Magnaporthe oryzae, a fungal pathogen of rice blast, is the most devastating rice pathogen and causes a destructive decrease in rice production in epidemic years. MoHrip2, a novel elicitor isolated from M. oryzae, is an exocrine protein. In our previous work, we showed that MoHrip2 causes necrotic lesions and triggers early signaling events in the tobacco leaf defense system, and we showed that MoHrip2 also enhanced resistance to M. oryzae in rice. Although, the MoHrip2 amino acid sequence showed up to 70% similarity to several specific plant fungal pathogen proteins, the specific function of both MoHrip2 and proteins with similar sequences are unknown.

In this study, we solved the crystal structure of MoHrip2 by X-ray crystallography using the single-wavelength anomalous dispersion (SAD) method. There were two identical protein molecules in an asymmetric unit, and only one monomer is shown. The overall architecture is a β-barrel consisting of 11 β-sheets and a very short α-helix. The short helix was located between the β9 and β10 sheet. MoHrip2 contains six cysteines that are involved in three intramolecular disulfide bridges, which occur between cysteines 27 and 151, 116 and 140, and 121 and 129. On the basis of the crystal structure, MoHrip2 showed a high similarity to the three-dimensional structure of a large family of proteins containing a thaumatin-like domain despite the low homology of their primary sequences. Of these proteins, we were interested in xylanase inhibitor TL-XI, to which MoHrip2 was most similar in three-dimensional structure. The 14 amino acid residues located in the middle region form the functional region responsible for the HR and the disease-resistance induction of the MoHrip2 elicitor. These 14 residues include a β-strand within a β-barrel and part of two neighboring loops. During the process of HR induction when interacting with its target, MoHrip2 might undergo local conformational changes around this stretch, especially in the loop regions, to expose active residues necessary for function.

>[2x]SNAQQAIVHNNCQDTVYVQSFPYDGSATGPLTTLQAGQTFSEDFRKSGSTVKVSKTKTLTSPMFIGYSFSSNPDYGYYELSSEWGNPFADKRVTLSPGAGCQDFNCAPNDAGCYSRPDMKKVYGCPLPINVEATLCA> SNAMIRFQPITTSDVQHYKFMEELLVESFPPEEYRELEHLREYTDRIGNFHNNIIFDDDLPIGFITYWDFDEFYYVEHFATNPALRNGGYGKRTLEHLCEFLKRPIVLEVERPVEEMAKRRINFYQRHGFTLW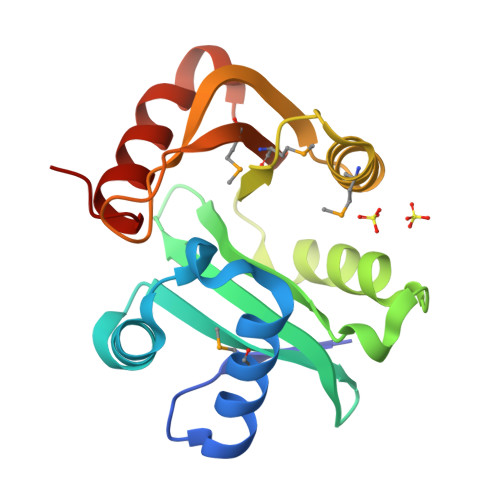EKDYYQPPYKEGDDFLPMYLMVHGNLDAEKDYEGIRHKLHTIVYGVKE2-(2,6-dimethylpyridin-4-yl)-5-(piperidin-4-yl)-3-(propan-2-yl)-1H-indole 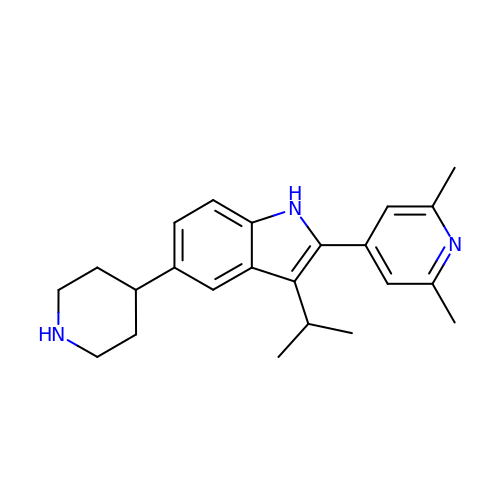| C23 H29 N3 | XSXCQWXAFRASGU-UHFFFAOYSA-N>PCTDSLIKVDMRTISFDIPPQEVLTKDSVTISVDGVVYYRVQNATLAVANITNAD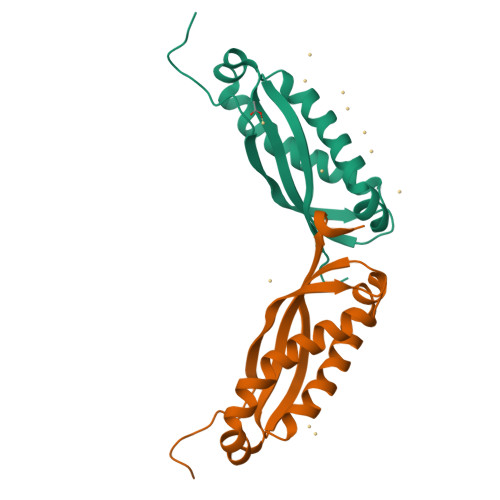SATRLLAQTTLRNALGTKNLSQILSDREEIAHHMQSTLDDATDDWGIKVERVEIKDVKLPVQLQRAMAAEAEA[2x]3,5,7,3',4'-PENTAHYDROXYFLAVONE | C15 H10 O7 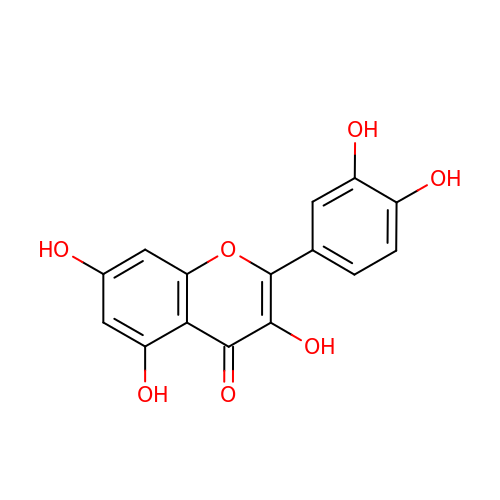| REFJWTPEDVJJIY-UHFFFAOYSA-N> SNATNTDTNSTNNSPNNTTNTTTNVTTTSDKNTIPIGIALAQTSNVALLGQEQVAGAKIAEKYFNDKGGVNGTPIKLIFQDTAGDEAGTINAFQTLINKDKVVGIVGPTLSQQAFSANPIAERAKVPVVGPSNTAKGIPEIGDYVA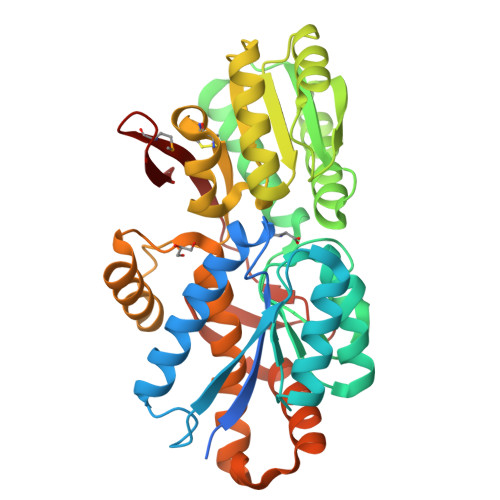RVSAPVSVVAPNSVKAALKQNPNIKKVAVFFAQNDAFSKSETEIFQQTVKDQGLELVTVQKFQTTDTDFQSQATNAINLKPDLVIISGLAADGGNLVRQLRELGYQGAIIGGDGLNTSNVFAVCKALCDGVLIAQAYSPEYTGEINKAFRQAYVDQYKKEPPQFSAQAFAAVQVYVESLKALDTKNKVSKIQLPELRTELNKQLLTGKYNTPLGEISFTPIGEVVQKDFYVAQIKMEKDGSQGKFTFLK> MSDGVEVKNITFKLGMYLTVGGVVNSNANRFSINV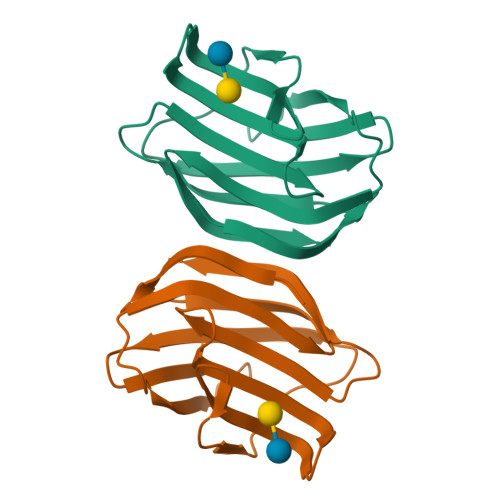GESTDSIALHIDHRFSYGADQNTIVLNSMVDDGWQQEQRSKNFPFTAGEHFQITITFDIDTFYIQLPDGHKVEFPNRHGDEAFNFIYLAGDARLTFVRLE> GAMAMHPMLNIAVRAARKAGNLIAKNYETPDAVEASQKGSNDFVTNVDKAAEAVIIDTIRKSYPQHTIITEESGELEGTDQDVQWVIDPLDGTTNFIKRLPHFAVSIAVRIKGRTEVAVVYDPMRNELFTATRGQGAQLNGYRLRGSTARDLDGTILATGFPFKAKQYATTYINIVGKLFNECADFRRTGSAALDLAYVAAGRVDGFFEIGLRPW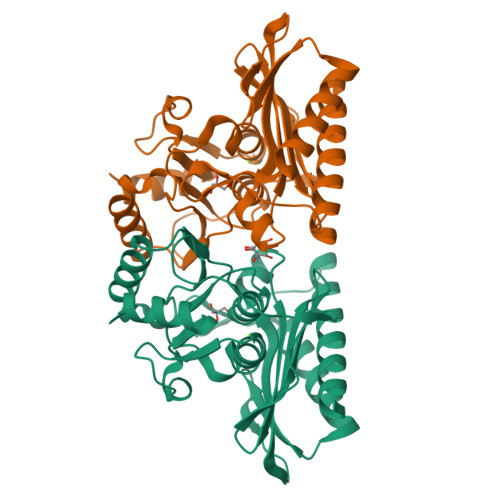DFAAGELLVREAGGIVSDFTGGHNYMLTGNIVAGNPRVVKAMLANMRDELSDALKR(2~{R},3~{R},4~{S},5~{R})-2-(6-aminopurin-9-yl)-5-[3-(6-azanyl-9~{H}-purin-8-yl)prop-2-ynoxymethyl]oxolane-3,4-diol 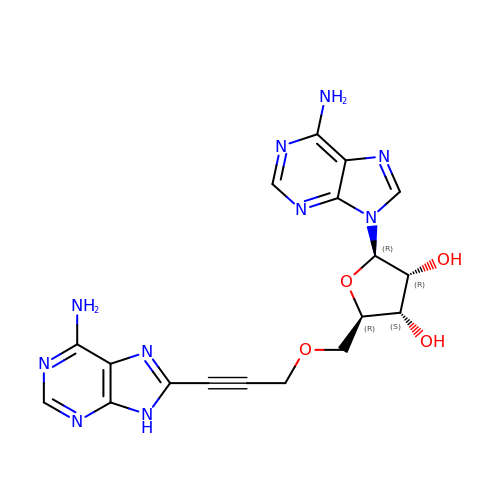| C18 H18 N10 O4 | BVXWUAMSMQSLCT-IKGPEZKQSA-N> SAAVESFVTKQLDLLELERDAEVEERRSWQENISLKELQSRGVCLLKLQVSSQRTGLYGRLLVTFEPRRYGSAAALPSNSFTSGDIVGLYDAANEGSQLATGILTRVTQKSVTVAFDESHDFQLSLDRENSYRLLKLANDVTYRRLKKALIALKKYHSGPASSLIEVLFGRSAPSPASEIHPLTFFNTCLDTSQKEAVLFALSQKELAIIHGPPGTGKTTTVVEIILQAVKQGLKVLCCAPSNIAVDNLVERLALCKQRILRLGHPARLLESIQQHSLDAVLARSDSAQIVADIRKDIDQVFVKNKKTQDKREKSNFRNEIKLLRKELKEREEAAMLESLTSANVVLATNTGASADGPLKLLPESYFDVVVIDECAQALEASCWIPLLKARKCILAGDHKQLPPTTVSHKAALAGLSLSLMERLAEEYGARVVRTLTVQYRMHQAIMRWASDTMYLGQLTAHSSVARHLLRDLPGVAATEETGVPLLLVDTAGCGLFELEEEDEQSKGNPGEVRLVSLHIQALVDAGVPARDIAVVSPYNLQVDLLRQSLVHRHPELEIKSVDGFQGREKEAVILSFVRSNRKGEVGFLAEDRRINVAVTRARRHVAVICDSRTVNNHAFL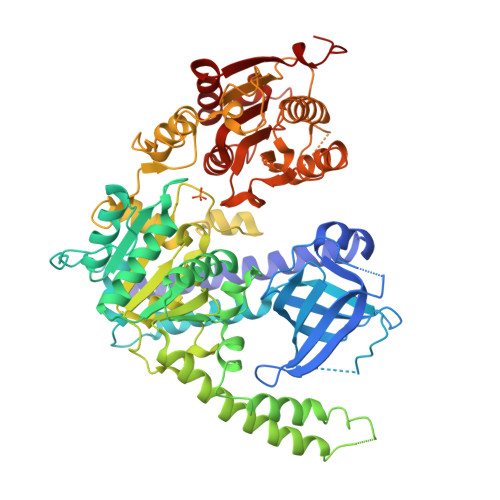KTLVEYFTQHGEVRTAFEYLDDIVP> 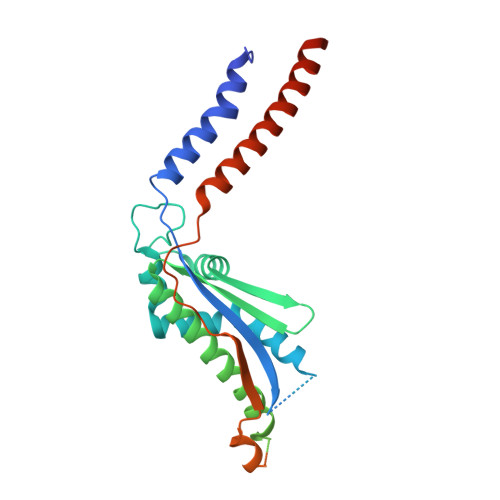MGKIHMKLVSRLTAKRLQWALVYLPMLVATVYFLVFSADRYVSESVITVRQTSSNAPTGGMSGAALLLAGLTPASREDTCYLQTYIHSMGLLQKLDQQLKLREHFGTPLRDPLFRLWGGTSQEWFLEYYRSRVEVLMDDICGLLTVRVQGFEPEFAQALNRAILEESERFVNELSHRMAREQGQFAEAELERATARLQEAKRQLIAFQAKHKLLDPLAQAQATGTLTAELQAALTRQEAELRNALTYLNEDSYQVKALRSQINALRQQIDEERLRATAGKNGDRINAVAAEFHDLQLQVGFAEDAYKLALAAVESARIEATRKLKSLVVVEPPVLPEIAEYPRRWYNLATLLVVCCLIYGVVSLVVATIRDHQDGSGSGSHHHHHHHHHH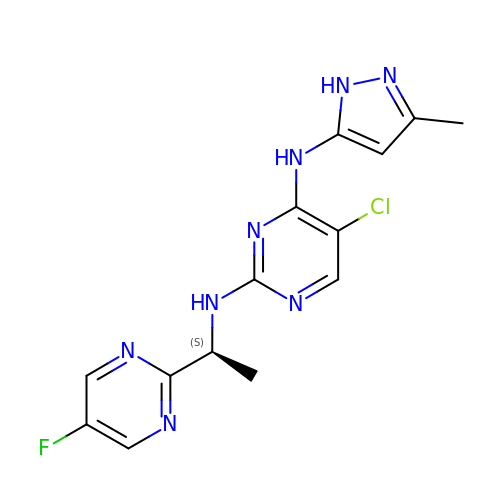5-CHLORO-N2-[(1S)-1-(5-FLUOROPYRIMIDIN-2-YL)ETHYL]-N4-(5-METHYL-1H-PYRAZOL-3-YL)PYRIMIDINE-2,4-DIAMINE | C14 H14 Cl F N8 | PDOQBOJDRPLBQU-QMMMGPOBSA-N>[4x]LWDYDFLQSLGRHSSVTEEHVGLAEKLKGEVKSLITGPMEPLAKLEFIDSVRRLGLKYQFETEMKEALANISKDGYDSWWVDNLRATALRFRLLRENGIFVPQDVFERFQNKETGKFKNELCEDVKGLLNLYEASFLGWEGEDILDEARTFSTAQLKNVEKKISSPNLAKIVHHALDLPLHWRAIRYEARWFIDIYEDEEDMNPT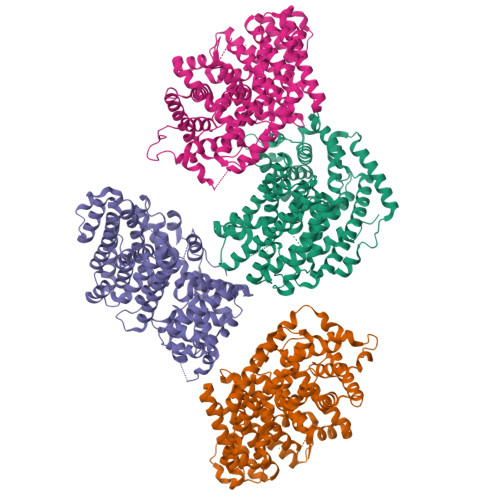LLKYAKLDFNIVQSFHQAEIGRLARWWVGTGLDKLPFARNGLIQSYMYAIGMLFEPHLGEVREMEAKVGALISTIDDVYDVYGTMEELELFTDITERWDINRVDQLPRNIRMPLLTMFNTSNDIGYWALKERGFNGIPYTAKVWADQLKSYTKEAKWFHEGHKPTLEEYLENALVSIGFPNLLVTSYLLTVDNPTKEKLDYVDSLPLFVRASCILCRIINDLGTSPDEMERGDNLKSIQCYMNETGASQEVAREHIEGLVRMWWKRLNKCLFEPSPFTEPFLSFTINVVRGSHFFYQYGDGYGNAESWTKNQGMSVLIHPITL>MKITVIGAGNVGATTAFRIADKKLARELVLLDVVEGIPQGKGLDMYETGPVGLFDTKITGSNDYADTADSDIVIITAGLPRKPGMTREDLLMKNAGIVKEVTDNIMKHSKNPIIIVVSNPLDIMTHVAWVRSGLPKERVIGMAGVLDAARFRSFIAMELGVSMQDINACVLGGHGDAMV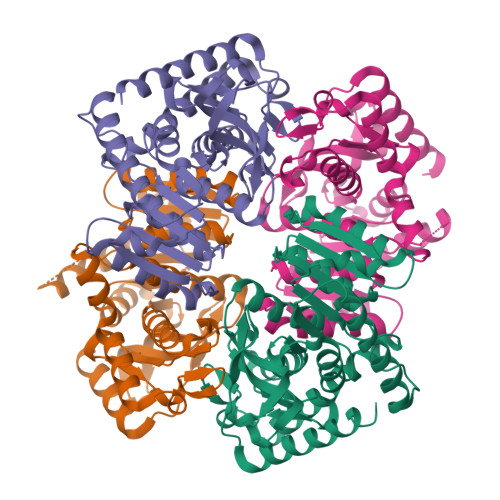PVVKYTTVAGIPISDLLPAETIDKLVERTRNGGAEIVEHLKQGSAFYAPASSVVEMVESIVLDRKRVLPCAVGLEGQYGIDKTFVGVPVKLGRNGVEQIYEINLDQADLDLLQKSAKIVDENCKMLESTIG[4x]ALPHA-RIBAZOLE-5'-PHOSPHATE | C14 H19 N2 O7 P | 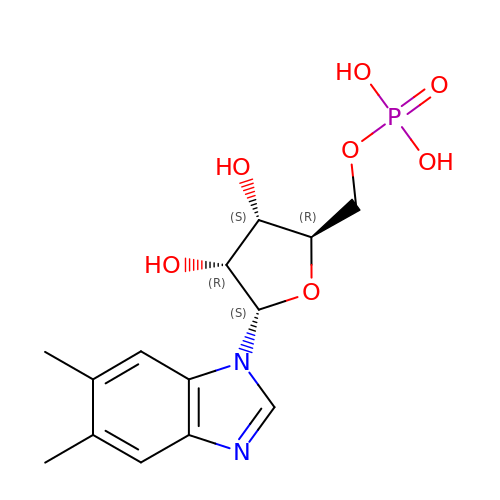ZMRGXEJKZPRBPJ-SYQHCUMBSA-N> SGSMEIRVRV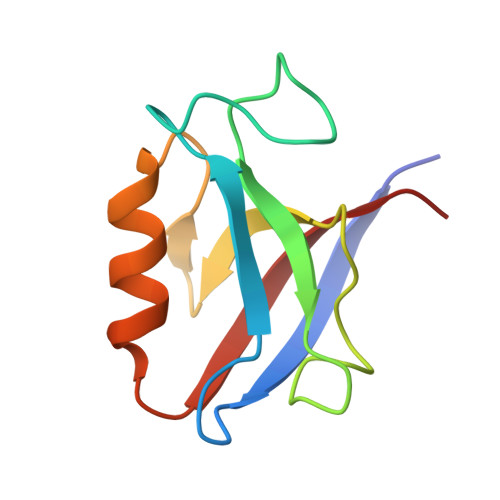EKDPELGFRIAGGVGGRGNPFRPDDDGIFVTRVQPEGPASKLLQPGDKIIQANGYSFINIEHGQAISLLKTFQNTVELIIVREV Lectins are carbohydrate binding proteins unrelated to immunoglobulins that display no enzymatic activity towards the recognized sugars. Lectins purified from seeds of the Diocleinae subtribe exhibit a high degree of sequence identity notwithstanding that they show very distinct biological activities. In the present study, we used mass spectrometry to determine the amino acid sequence of a lectin from Canavalia boliviana seeds and solved its crystal structure in complex with Xman and the dimannosides Man(α1-3)Man(α1-O)Me and Man(α1-4)Man(α1-O)Me. Furthermore, we characterized the anti-inflammatory properties of Cbol, adding more data to the repertoire of wide biological activities displayed by this group of lectins, despite their highly identical sequence.

Other than in the carbohydrate-binding region, the complexes do not present any significant structural differences when compared to the unbound protein.

>[2x]ADTIVAVELDTYPNTDIGDPSYPHIGIDIKSVRSKKTAKWNMQNGKVGTAHIIYNSVGKRLSAVVSYPNGDSATVSYDVDLDNVLPEWVRVGLSATTGLYKETNTILSWSFTSKLKSNSTHETNALHFMFNQFSKDQKDLILQGDATTGRDGNLELTRVSSNGSPQGSSVGRALFYAPVHIWESSAVVASFDATFTFLIKSSDSHPADGIAFFISNIDSSIPSGSTGRLLGLFPDAN>MDVKVQYLCENTQTSQQEIKGKF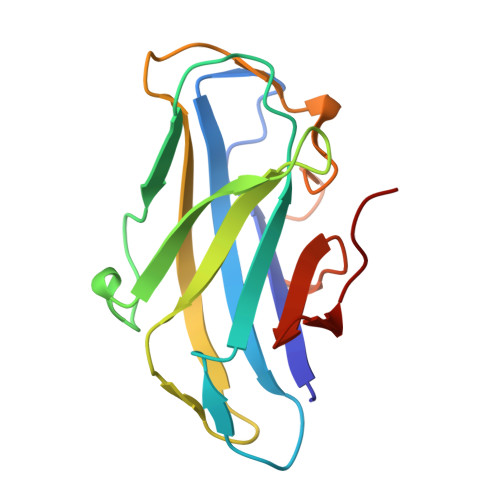NIVNTGNRDYSLKDIVLRYYFTKEHNSQLQFICYYTPIGSGNLIPSFGGSGDEHYLQLEFKDVKLPAGGQTGEIQFVIRYADNSFHDQSNDYSFDPTIKAFQDYGKVTLYKNGELVWGTPPG[4x]>[2x]GLGGLERFCSPGKGRGLRALQPFQVGDLLFSCPAYAYVLTVNERGNHCEYCFTRKEGLSKCGRCKQAFYCNVECQKEDWPMHKLECSPMVVFGENWNPSETVRLTARILAKQKIHPERTPSEKLLAVKEFESHLDKLDNEKKDLIQSDIAALHHFYSKHLEF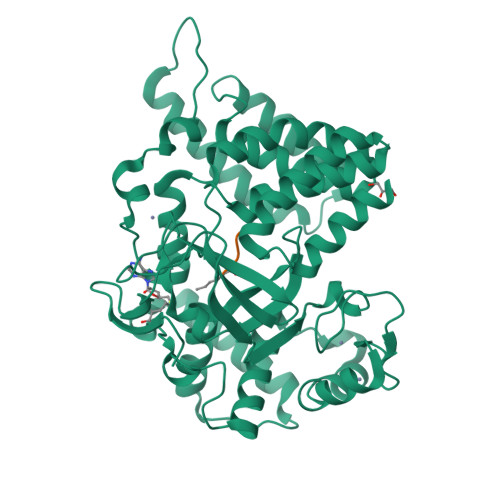PDNDSLVVLFAQVNCNGFTIEDEELSHLGSAIFPDVALMNHSCCPNVIVTYKGTLAEVRAVQEIKPGEEVFTSYIDLLYPTEDRNDRLRDSYFFTCECQECTTKDKDKAKVEIRKLSDPPKAEAIRDMVRYARNVIEEFRRAKHYKSPSELLEICELSQEKMSSVFEDSNVYMLHMMYQAMGVCLYMQDWEGALQYGQKIIKPYSKHYPLYSLNVASMWLKLGRLYMGLEHKAAGEKALKKAIAIMEVAHGKDHPYISEIKQEIESH;>KLLSKRG[2x]> SGVDDDMACH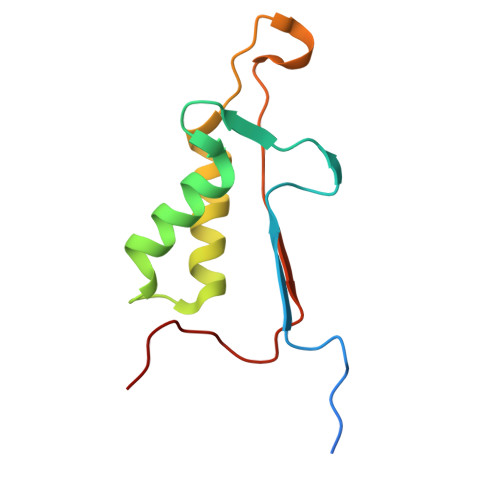KIPVEADFLYAYSTAPGYYSWRNSKDGSWFIQSLCAMLKQYADKLEFMHILTRVNRKVATEFESFSFDATFHAKKQIPCIVSMLTKELYFYHH> IT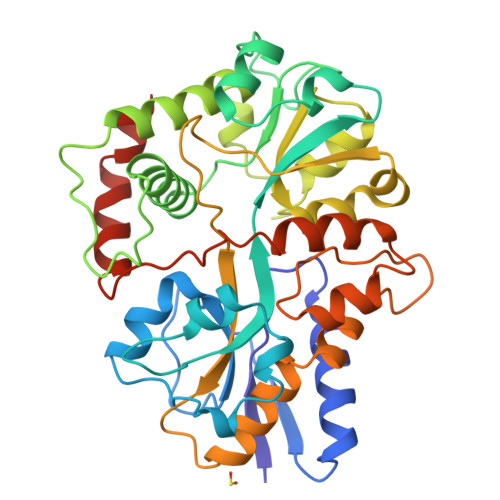LKVAIYPYVPDPARFQAAVLDQWQRQEPGVKLEFTDWDSYSADPPDDLDVFVLDSIFLSHFVDAGYLLPFGSQDIDQAEDVLPFALQGAKRNGEVYGLPQILCTNLLFYRKGDLKIGQVDNIYELYKKIGTSHSEQIPPPQNKGLLINMAGGTTKASMYLEALIDVTGQYTEYDLLPPLDPLNDKVIRGLRLLINMAGEKPSQYVPEDGDAYVRASWFAQGSGRAFIGYSESMMRMGDYAEQVRFKPISSSAGQDIPLFYSDVVSVNSKTAHPELAKKLANVMASADTVEQALRPQADGQYPQYLLPARHQVYEALMQDYPIYSELAQIVNKPSNRVFRLGPEVRTWLKDAKQVLPEALGLTDVSSLAS> MMNFILVLLIVAMIGTILVSESKYLFSKPVCKNCGVK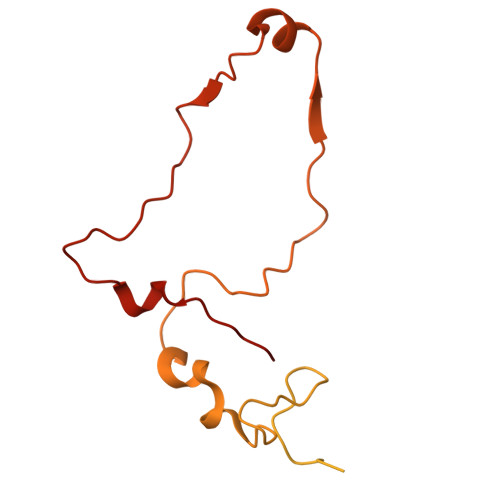AVTLPVDISAGKLAKVAEAVKKQTEEIKTLLKQKQSAPKAPELTNPIEHIKASTTVVSGANGLENVIDEDLPFSDFKGVPVAETTVEGMIKGIRPPTYADPRVMNPALAAAPVQFSDPTQFGTFGVTDDVSPAFSTEDKIPKTNAKISSDISVEGYENSYDANGARLVMDGKVVKSECQLPSYQIRNSKHHTQLPMRSLNEPPPMVEDLVDESLFEGLQGYPVDEKLDLLTPPGTATPSSEWAAINYGLTNN> MPDFVKPAPIGVGIQYNPEILDWFPFEDIQVDILEILLDNIMAPMDGPQIIKPSAQAMIERLGQKFTLLAHSNYGCDFGFSALEETAAVQRHVPLAKMLNSPWVANHCFYGDQSWLDIWSSPIQFSAAEVARCADRAQSLQTLYGMPLAHENAAYYLECPGAEMREAEFLARLVQRSGTFLHLDLHNIYTNHLNLKGFDLKDYMDTLPLDKVISVHLAGGSWHGGLYHDWHDACVPEPVWDLYEDLLSRAQPSAVI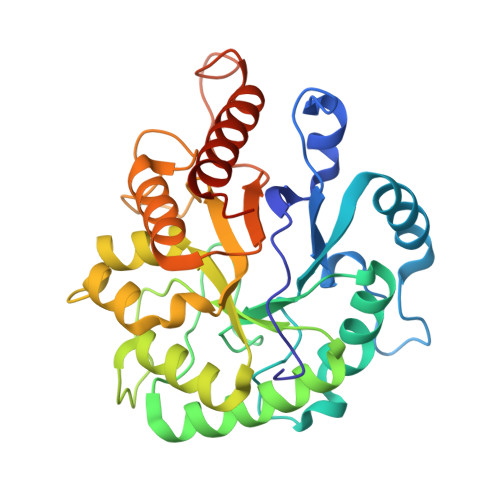LEYQGQAHHAQTRIMDASDESMIVRDVQRAQAIWSRYNRHPQERQYGS The iron-dependent regulator IdeR is the main transcriptional regulator controlling iron homeostasis genes in Actinobacteria, including species from the Corynebacterium, Mycobacterium and Streptomyces genera, as well as the erythromycin-producing bacterium Saccharopolyspora erythraea. IdeR is an OCS from the DtxR (Diphtheria toxin repressor) family of transcriptional regulators which typically consist of three domains: an N-terminal DNA-binding winged helix-turn-helix (wHTH) motif, followed by a dimerization interface that contains most of the metal-binding residues, and a C-terminal SH3-like domain (21–23). The main function of IdeR is to repress the expression of iron uptake genes when the intracellular iron levels are sufficient. When iron levels are sufficient for iron ions to occupy the IdeR metal-binding sites, the regulator is activated and recognizes a highly conserved 19-bp sequence located in the promoter region of its target genes.

The first two putative IdeR binding sites in the cluster (C10S1 and C10S2) can be found in the intergenic region between genes SACE_2689 and SACE_2690. We also determined the crystal structure of the Co2+-activated complex of IdeR and C10S1 DNA. The structure of this complex does not display any significant differences compared to the complexes with the consensus sequence. The C10S1 sequence differs from the consensus in position 3 of the first repeat, and positions 2 and 4 of the second repeat. These differences affect the interactions with one subunit of each IdeR dimer. Specifically, the vdW interactions with Pro39 and Ser37 of one IdeR subunit, and the vdW interactions with Pro39 and Thr40 of the IdeR subunit bound to the neighboring major groove are affected. However, the only notable differences regarding these distance-dependent interactions are the absence of the thymine methyl group in position 3 of the first repeat and the presence of a thymine methyl group in position 2 of the second repeat, as the distances between Pro39 and the fourth base pair are very similar regardless of the nature of the bases. The water-mediated hydrogen bond with Glu43 and Pro39 should not be affected by the different base in position 2 of the second repeat, but the water molecule, though likely present, was not clearly observed in the electron density and was not modelled. Despite these differences, IdeR binds to the C10S1 sequence in the same way as to the consensus sequence.

>[6x]GHMNDLIDTTEMYLRTIYDLEEEGVVPLRARIAERLEQSGPTVSQTVARMERDGLLTVAEDRHLELTKAGRARAISVMRKHRLAERLLVDVIGLEWEQVHLEACRWEHVMSEAVERKLVKLLGNPTTSPYGNPIPGLDELGVGDSVEPVDTDLRRVDEVARSGGGRALVCRIAEHVQLDPDLMSELKKVGVVPGNEIDIVAVAGVNKPIQVQGSEGGTQLQPGIAHAVMVRVK> GAGCAGACGAG;> ACCCCACT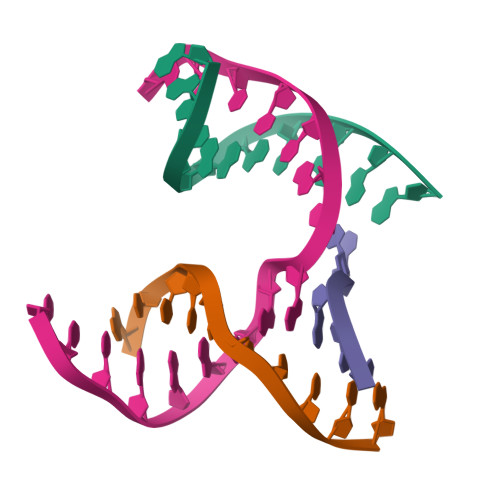CA;> CTGGT;> TCTGAGTGGCGTCTGC> TKEGYGKHITSMHVRNIFNQGNQVIRNIVKQQRYELLDFTGTEAGTTNLPKIIPYQCIWWRGLQNAANVNQTINNMIALNTISYGVRFLKAKLCIEVYAVTRKRLIQTGATSYYTDDFEQGQNLFIGWADRKAESIPITTPADLDETKLTVANTTLFDANNDNITKEEVPTREKWCHTWDLDVLNHNYLWE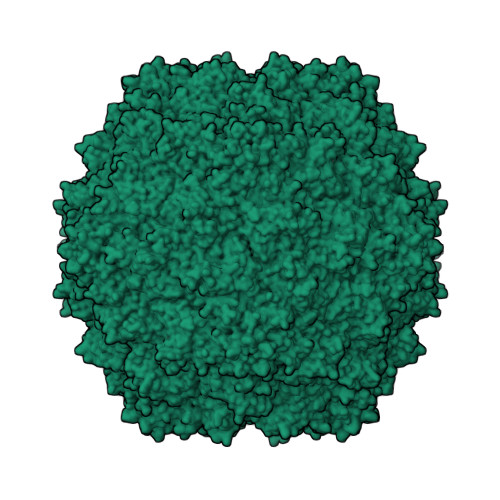PNNLDSQWTLIPGAQAVQPTATPIGPTYQEIVIATKAIGANESALVTTIQDRRSYPRLMLSQPQIKDETDTMKFKYQIRISTELEMEHHIKPDIANPWLTRQTLPLPALSGDGTTRYVPCVPYETHVSQRNWNHVGEYL>MRIVEVYSHLNGLEYIQVHLPHIWEEIQEIIVSIDAEACRTKESKEKTKQGQILYSPVALNEAFKEKLEAKGWKESRTNYYVTADPKLIRETLSLEPEEQKKVIEAAGKEALKSYNQTDFVKDRVAIEVQFGKYSFVAYDLFVKHMAFYVSDKIDVGVEILPMKELSKEMSSGISYYEGELYNVIRQGRGVPAVPLVL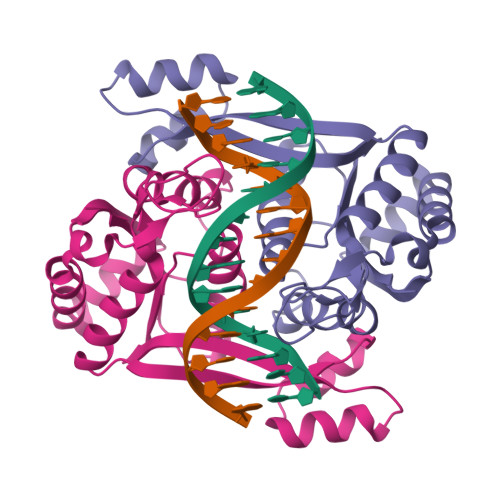IGIAP[2x]> QDADKLPHTKVTLVAPPQVHPHEQATKSGPKVVEFTMTIEEKKMVIDDKGTTLQAMTFNGSMPGPTLVVHEGDYVQLTLVNPATNAMPHNVDFHGATGALGGAKLTNVNPGEQATLRFKADRSGTFVYHCAPEGMVPWHVVSGMSGTLMVLPRDGLKDPQGKPLHYDRAYTIGEFDLYIPKGPDGKYKDYATLAESYGDTVQVMRTLTPSHIVFNGKVGALTGANALTAKVGETVLLIHSQANRDTRPHLIGGHGDWVWETGKFANPPQRDLETWFIRGGSAGAALYTFKQPGVYAYLNHNLIEAFELGAAGQIKV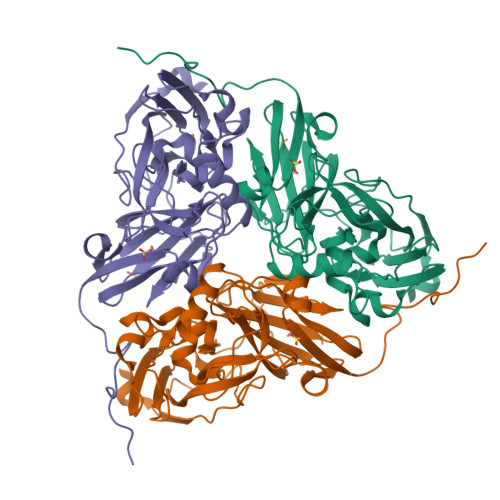EGKWNDDLMKQIKAPAPIPR>SVKNETVKLSVGTVS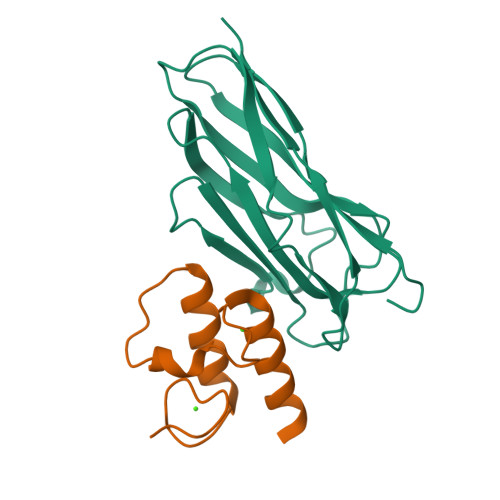GNPGDTVKVPVTISQVSTPVGLICMDISYDASKFTVKDVLPNTDLVKDTDNYSFIVNTSTPGKISITFTDPTLANYPISVDGILAYLDFIINSNATAGDSALTVDPATLIVADENDKDIKDAASNGKITVTGSAP[2x];>[2x]SNTILGDLNDDGVVNGDDIVMMRQYLAGKTVSGIDKNALDINGDGAVNGRDLMELIKKVSNN A key component, the RNA-dependent RNA polymerase [(RdRp), also known as nsp12], catalyzes the synthesis of viral RNA and thus plays a central role in the replication and transcription cycle of COVID-19 virus, possibly with the assistance of nsp7 and nsp8 as cofactors. Therefore, nsp12 is considered a primary target for nucleotide analog antiviral inhibitors such as remdesivir, which shows potential for the treatment of COVID-19 viral infections. The structure of the COVID-19 virus nsp12 contains a right-hand RdRp domain (residues S367 to F920) and a nidovirus-specific N-terminal extension domain (residues D60 to R249) that adopts a nidovirus RdRp-associated nucleotidyltransferase (NiRAN) architecture. The polymerase domain and NiRAN domain are connected by an interface domain (residues A250 to R365).

To inform drug design, we determined the structure of nsp12, in complex with its cofactors nsp7 and nsp8, by cryo–electron microscopy (cryo-EM) using two different protocols: one in the absence of dithiothreitol (DTT) and the other in the presence of DTT. After the collection and processing of 7994 micrograph movies, we obtained a 2.9-Å resolution three-dimensional reconstruction of an nsp12 monomer in complex with one nsp7-nsp8 pair and an nsp8 monomer, as was previously observed for SARS-CoV. The polymerase domain adopts the conserved architecture of the viral polymerase family and is composed of three subdomains: a fingers subdomain (residues L366 to A581 and K621 to G679), a palm subdomain (residues T582 to P620 and T680 to Q815), and a thumb subdomain (residues H816 to E920). Motif A, composed of residues 611 to 626 (TPHLMGWDYPKCDRAM), contains the classic divalent-cation–binding residue D618, which is conserved in most viral polymerases including hepatitis C virus (HCV) ns5b (residue D220) and poliovirus (PV) 3Dpol (residue D233). Motif C [residues 753 to 767 (FSMMILSDDAVVCFN)] contains the catalytic residues [759 to 761 (SDD)] in the turn between two β strands. The NTP entry channel is formed by a set of hydrophilic residues, including K545, R553, and R555 in motif F. The RNA template is expected to enter the active site composed of motifs A and C through a groove clamped by motifs F and G. Motif E and the thumb subdomain support the primer strand. The product-template hybrid exits the active site through the RNA exit tunnel at the front side of the polymerase. The catalytic metal ions, which are observed in several structures of viral polymerases that synthesize RNA, are not observed in this work in the absence of primer-template RNA and nucleoside triphosphates (NTPs). Overall, we found that the nsp12 of COVID-19 virus has the highest similarity with the apo state of ns5b.

> SADAQSFLNRVCGVSAARLTPCGTGTSTDVVYRAFDIYNDKVAGFAKFLKTNCCRFQEKDEDDNLIDSYFVVKRHTFSNYQHEETIYNLLKDCPAVAKHDFFKFRIDGDMVPHISRQRLTKYTMADLVYALRHFDEGNCDTLKEILVTYNCCDDDYFNKKDWYDFVENPDILRVYANLGERVRQALLKTVQFCDAMRNAGIVGVLTLDNQDLNGNWYDFGDFIQTTPGSGVPVVDSYYSLLMPILTLTRALTAESHVDTDLTKPYIKWDLLKYDFTEERLKLFDRYFKYWDQTYHPNCVNCLDDRCILHCANFNVLFSTVFPPTSFGPLVRKIFVDGVPFVVSTGYHFRELGVVHNQDVNLHSSRLSFKELLVYAADPAMHAASGNLLLDKRTTCFSVAALTNNVAFQTVKPGNFNKDFYDFAVSKGFFKEGSSVELKHFFFAQDGNAAISDYDYYRYNLPTMCDIRQLLFVVEVVDKYFDCYDGGCINANQVIVNNLDKSAGFPFNKWGKARLYYDSMSYEDQDALFAYTKRNVIPTITQMNLKYAISAKNRARTVAGVSICSTMTNRQFHQKLLKSIAATRGATVVIGTSKFYGGWHNMLKTVYSDVENPHLMGWDYPKCDRAMPNMLRIMASLVLARKHTTCCSLSHRFYRLANECAQVLSEMVMCGGSLYVKPGGTSSGDATTAYANSVFNICQAVTANVNALLSTDGNKIADKYVRNLQHRLYECLYRNRDVDTDFVNEFYAYLRKHFSMMILSDDAVVCFNSTYASQGLVASIKNFKSVLYYQNNVFMSEAKCWTETDLTKGPHEFCSQHTMLVKQGDDYVYLPYPDPSRILGAGCFVDDIVKTDGTLMIERFVSLAIDAYPLTKHPNQEYADVFHLYLQYIRKLHDELTGHMLDMYSVMLTNDNTSRYWEPEFYEAMYTPHTVLQHHHHHHHHHH;>[2x]AIASEFSSLPSYAAFATAQEAYEQAVANGDSEVVLKKLKKSLNVAKSEFDRDAAMQRKLEKMADQAMTQMYKQARSEDKRAKVTSAMQTMLFTMLRKLDNDALNNIINNARDGCVPLNIIPLTTAAKLMVVIPDYNTYKNTCDGTTFTYASALWEIQQVVDADSKIVQLSEISMDNSPNLAWPLIVTALRANSAVKLQ;> SKMSDVKCTSVVLLSVLQQLRVESSSKLWAQCVQLHNDILLAKDTTEAFEKMVSLLSVLLSMQGAVDINKLCEEMLDNRATLQ3-METHYLBUTAN-1-AMINE | C5 H13 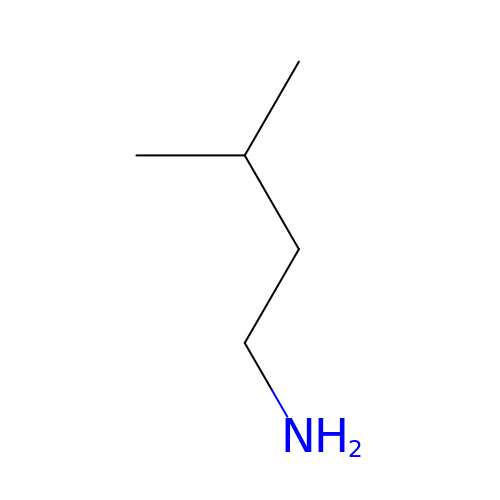N | BMFVGAAISNGQNM-UHFFFAOYSA-N> RLGEVFVLDEEEIRIIQTEAEGIGPENVLNASYSKLKKFIESADGFTNNSYGATFSFQPYTSIDEMTYRHIFTPVLTNKQISSIT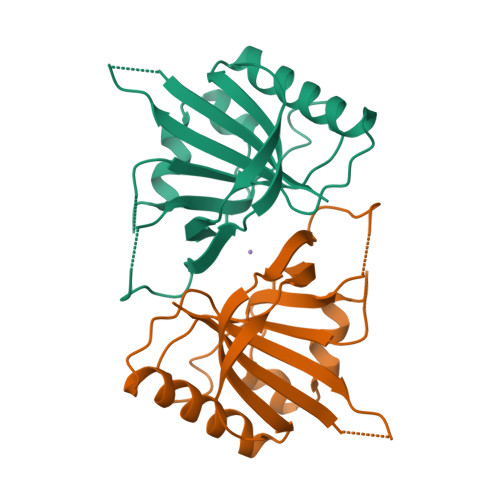PDMEITTIPKGRYACIAYNFSPEHYFLNLQKLIKYIADRQLTVVSDVYELIIPIHYSPKKQEEYRVEMKIRILE>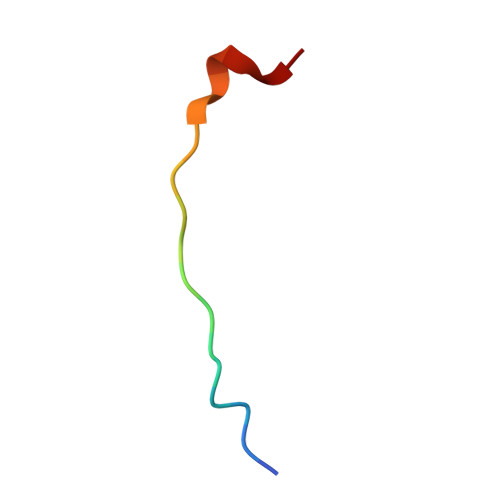 DEEGGGEEDQDFDLSQLH> SMKSVKYISNMSKQEKGYRVYVNVVNEDTDKGFLFPSVPKEVIENDKIDELFNFEHHKPYVQKAKSRYDKNGIGYKIVQLDEGFQKFIELNKEKMKENL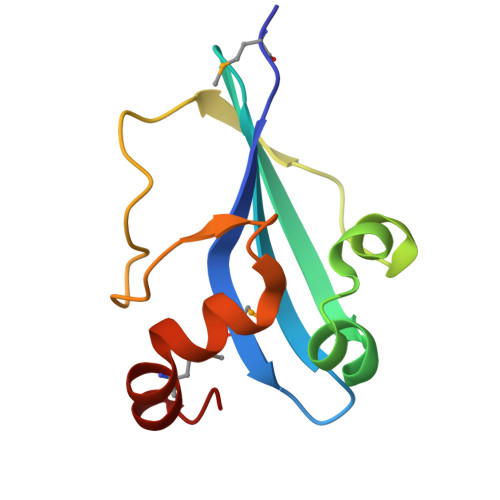DY>MNPDDIVVLVGRKKSGKSYLIKHYFIPVLKAHKISYIIDDHNLLRSGSEYSKFGYNATSLSDIVSKQYVVVYDRAKNDDFFEKLWQASKLHSKKYGTTVLIIDEAYYHFKYKQKVTPAIDEALHANRHAGLGLILSTQRVYDLMPIVYKQADLIIMFYTREPNELRWISKYISAEAAEKVKTLKQY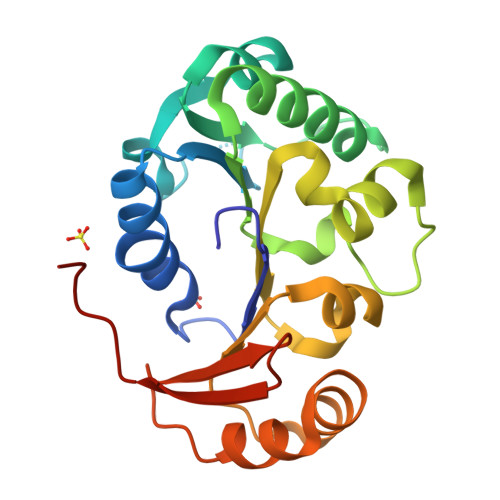HFLIYDVNSQTIKIHKPILEHHHHHH[3x]>MSKEVLEKELFEMLDEDVRELLSLIHEIKIDRITGNMDKQKLGKAYFQVQKIEAELYQLIKVSHH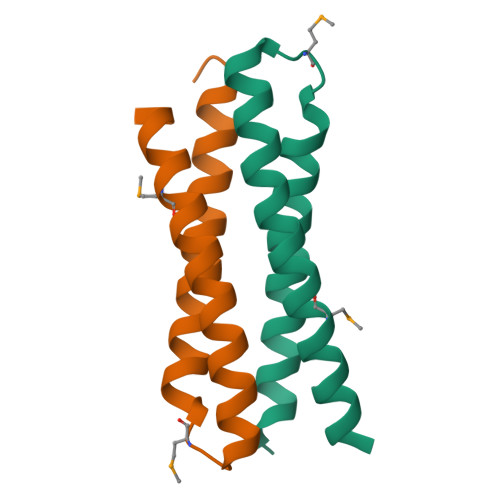HHHH[4x]> MNTSFGSVVPSTNFNFFKGHGNNDNTSANSTVNNSNFFLNSNETKPSKNVFMVHSTSQKKSQQPLQNLSHSPSYTENKPDKKKKYMINDAKTIQLVGPLISSPDNLGFQKRSHKARELPRFLINQEPQLEKRAFVQDPWDKANQEKMISLEESIDDLNELYETLKKMRNTERSIMEEKGLVDKADSAKDLYDAIVFQGTCLDMCPTFERSRRNVEYTVYSYEKNQPNDKKASRTKALKVFARPAAAAAPPLPSDVRPPHILVKTLDYIVDNLLTTLPESEGFLWDRMRSIRQDFTYQNYSGPEAVDCNERIVRIHLLILHIMVKSNVEFSLQQELEQLHKSLITLSEIYDDVRSSGGTCPNEAEFRAYALLSKIRDPQYDENIQRLPKHIFQDKLVQMALCFRRVISNSAYTERGFVKTENCLNFYARFFQLMQSPSLPLLMGFFLQMHLTDIRFYALRAL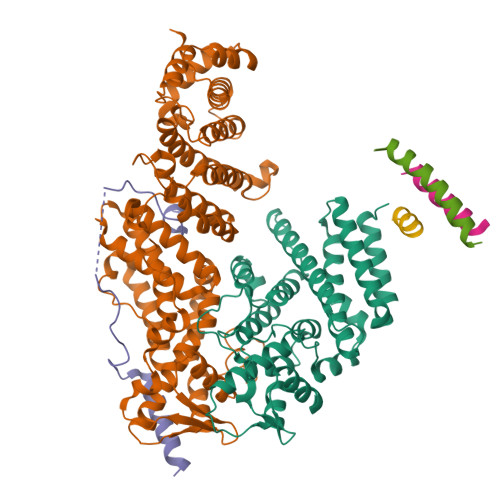SHTLNKKHKPIPFIYLENMLLFNNRQEIIEFCNYYSIEIINGDAADLKTLQHYSHKLSETQPLKKTYLTCLERRLQKTTYKGLINGGEDNLASSVYVKDPKKDRIPSIADQSFLMENFQNNYNEKLNQNSSVKPQINTSPKRVATRPNHFPFSQESKQLPQISQSHTLSTNPLLTPQVHGDLSEQKQQQIKTVTDGGSPFVFDQSAQNSTVEASKAHMISTTSNGAYDEKLSSEQEEMRKKEEQRIEEEKTQLKKKQENADKQVITEQIANDLVKEVVNSSVISIVKREFSEANYRKDFIDTMTRELYDAFLHERLYLIYMDSRAELKRNSTLKKKFFEKWQASYSQAKKNRILEEKKREEIKLVSHQLGVPGFKKSTCLFRTPYKGNVNSSFMLSSSDKNLIFSPVNDEFNKFATHLTKISKLWRPLEMQSIYYDNLTKKFPSNSLTPANLFIYAKDWTSLSNRWILSKFNLQTAQDSKKFSNNIISSRIICIDDEYEPSDFSDLQLLIFNTGVTNPDIFDLEMKLKDDGEELIKLITGISLNTNICFSLLIIYWESAENTLSESTIKHLLKLNRISKNYSSVIERIDLMNLTEESPHKCLEDKLSEISHSYVYKLTERGKYDKTLRQKRSLAGIHSRSTQLQTTKDIDQKMKKMLEKEKNKYQQQIGERNTYAHLESHIDASPRSKKRKLPILLSTSHSSQFKTPLASRLNTSGSSTSPPLPSHLAMKFRKNSRVTSLHTVLPVSTPSHSNNIPAASFSGNNTTDIQSQQLIENQKSTSVYLNNVSERILGNQEICQTPINPVTPVLDGADQGKEDIPDSILELKILIDSVKKKVNND;> MDMANQLLDELAHGNFSHLTLNLSQNGREIAILQKQLTGFDDKQLETFVEQHPAMPNDTRFKIMCTSFLNYARDVDPWSAWSSSDLIFEFYQCLINCLINDNAPHIEMLIPVATRETEFIINLAGKLDSFHLQLHTRSHQFLSHISSILSRLFNSIKPPRGNASSTNIPGKQRILLYLVNKLNNIYFRIESPQLCSNIFKNFQPKSMLAHFNEYQLDQQIEYRYLLGRYYLLNSQVHNAFVQFNEAFQSLLNLPLTNQAITRNGTRILNYMIPTGLILGKMVKWGPLRPFLSQETIDNWSVLYKHVRYGNIQGVSLWLRQNERHLCARQLLIVLLEKLPMVTYRNLIKTVIKSWTTEWGQNKLPYSLIERVLQLSIGPTFEDPGAQEITIYNGIHSPKNVENVLVTLINLGLLRANCFPQLQLCVVKKTTMIQEIVPPVNERITKMFPAHSHVLW;> MSTDVAAAQAQSKIDLTKKKNEEINKKSLEEDDEFEDFPIDTWANGETIKSNAVTQTNIWEENWDDVEVDDDFTNELKAELDRYKRENQ>[4x]MQKQRTTSQWRELDAAHHLHPFTDTASLNQAGARVMTRGEGVYLWDSEGNKIIDGMAGLWCVNVGYGRKDFAEAARRQMEELPFYNTFFKTTHPAVVELSSLLAEVTPAGFDRVFYTNSGSESVDTMIRMVRRYWDVQGKPEKKTLIGRWNGYHGSTIGGASLGGMKYMHEQGDLPIPGMAHIEQPWWYKHGKDMTPDEFGVVAARWLEEKILEIGADKVAAFVGEPIQGAGGVIVPPATYWPEIERICRKYDVLLVADEVICGFGRTGEWFGHQHFGFQPDLFTAAKGLSSGYLPIGAVFVGKRVAEGLIAGGDFNHGFTYSGHPVCAAVAHANVAALRDEGIVQRVKDDIGPYMQKRWRETFSRFEHVDDVRGVGMVQAFTLVKNKAKRELFPDFGEIGTLCRDIFFRNNLIMRACGDHIVSAPPLVMTRAEVDEMLAVAERCLEEFEQTLKARGLA

The crystal structures and inhibitor complexes of two industrially important ω-aminotransferase enzymes from Pseudomonas aeruginosa and Chromobacterium violaceum have been determined in order to understand the differences in their substrate specificity. The two enzymes share 30% sequence identity and use the same amino acceptor, pyruvate; however, the Pseudomonas enzyme shows activity towards the amino donor β-alanine, whilst the Chromobacterium enzyme does not. Both enzymes show activity towards S-α-methylbenzylamine (MBA), with the Chromobacterium enzyme having a broader substrate range. It appears that the different rigidity of the protein scaffold contributes to the substrate specificity observed for the two ω-­aminotransferases.

Crystallization with a significant excess of cofactor (at least 5 mM) was required to obtain holoenzyme crystals at pH 8.5. The holoenzyme structure presented here has full occupancy of the cofactor in the active site, which forms the internal aldimine link to the active-site Lys288. C. violaceum Am:PyAT elutes with an apparent molecular mass of 100 kDa on a size-exclusion chromatography column, which corresponds to a dimer. This enzyme is found to be a dimer in the crystal, with the asymmetric unit containing one (apoenzyme and mCPP complex) or two (holoenzyme) dimers. Formation of the C. violaceum Am:PyAT holoenzyme dimer buries 5600 Å2, which equates to 28% of the solvent-accessible area of each subunit. Significant structural rearrangements accompany cofactor binding in C. violaceum (CV) Am:PyAT, as also described by Humble et al.. This includes unwinding of the α-helix (residues CV 317–322) to form a loop covering the PLP phosphate group. The N-terminus (up to residue 36), which is disordered in the apoenzyme structure, becomes ordered in the holoenzyme structure and occupies the position of the unwound helix. Residue CV Thr321, which is conserved among ATs, forms hydrogen bonds to the phosphate of the PLP through peptide and side-chain interactions in the holo­enzyme.> MAAYQVLIVGAGFSGAETAFWLAQKGVRVGLLTQSLDAVMM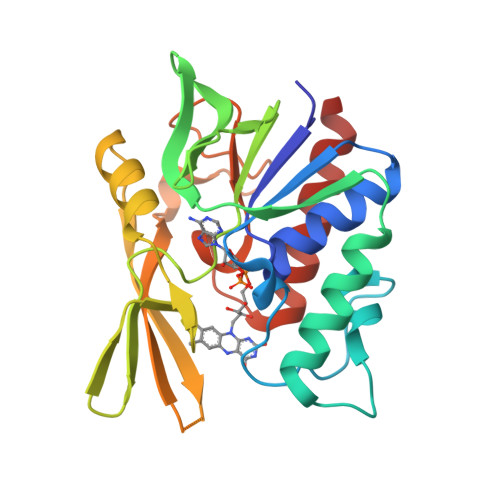PFLPPKPPFPPGSLLERAYDPKDERVWAFHARAKYLLEGLRPLHLFQATATGLLLEGNRVVGVRTWEGPPARGEKVVLAVGSFLGARLFLGGVVEEAGRLSEASYPDLLEDLSRLGFRFVEREGEVPETPSTPGYRVRYLAFHPEEWEEKTFRLKRLEGLYAVGLCVREGDYARMSEEGKRLAEHLLHELG> MESTALQQAFDTSQNNKAAWLQRKNELAAAEQEYLRLLSGEGRNVSRLDELRNIIEVRKWQVNQAAGRYIRSHEAVQHISIRDRLNDFMQQHGTALAAALAPELMGYSELTAIARNSAIQRACDALRE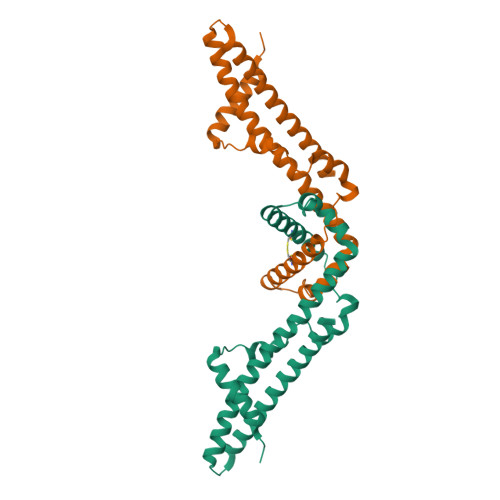ALLSWLAKGEKINYSAQDSDILTTIGFRPDVASVDDSREKFTPAQNMIFSRKSAQLASRQSV> MRVKHAVVLLMLISPLSWAGTMTFQFRNPNFGGNPNNGA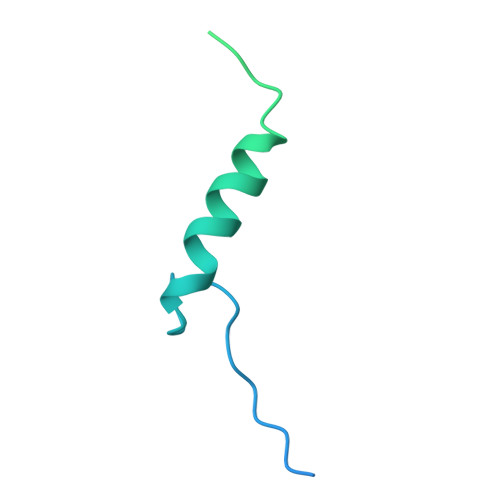FLLNSAQAQNSYKDPSYNDDFGIETPSALDNFTQAIQSQILGGLLSNINTGKPGRMVTNDYIVDIANRDGQLQLNVTDRKTGQTSTIQVSGLQNNSTDFHHHHHH3-isothiocyanatoprop-1-ene 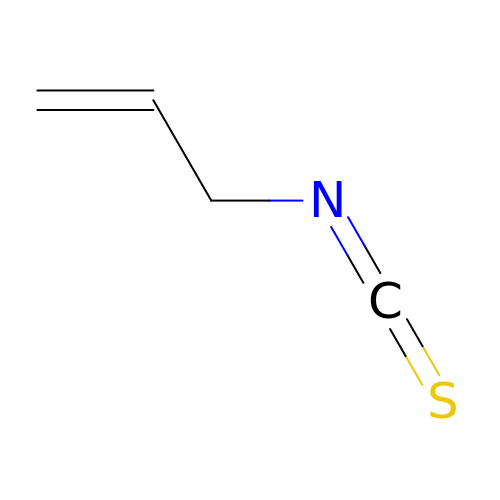| C4 H5 N S | ZOJBYZNEUISWFT-UHFFFAOYSA-N>[5x]GSHMGGIEVLDVKTGDDSITQIEAFLNPRMGVNDETNTWYGFSEQV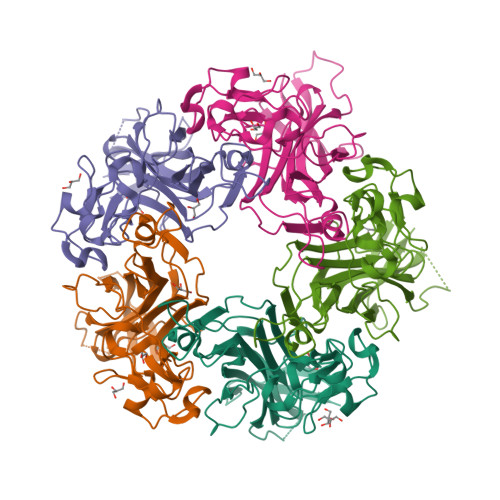TVATARETDRPPKEQMPYYSCARIPLPLLNEDMTCNTLLMWEAVSVKTEVIGSNTLMNVHDYMTRTDNGVGHPVVGSTYHMFAVGGEPLDLQGIQQSHLVQYPEGLIVPKSVTDVTAKIQCLDPSAKAKLDKDGKYPIETWSPDPSRNENTRYFGNYYGGLTTPPVLTFTNTVTTILLDENGVGPLCKGDGLFLSCCDVMGWFTAGSGTHQRFRGLPRYFNVQLRKRAVRN>GAEPGARPPRIRIKTGIEVLKEQNFKCLEGKRVGLITNPTGVDNHLISTIDILHEAPNVNLVALYGPEHGVRGDVHAGDKVDNANDSSTGLPVYSLYGKTRKPTPEMLKDIDVLVYDIQDIGCRSFTYISTMGVAMEAAAENNKEFIVLDRPNPIGGLKIEGNVVEDGYISFVSQFKIPYLYGLTCGELALMLNGEQMLSKPCNLHVVKMKGWKRKMDYVQTGLQWIPSSPHIPHPHSAFFYPVSGILGELGYMSIGVGYTIPFQMFAARWVEAEKLADNLNRLHLPGVIFRPMHLKPFYSVGKEEHLQGVQVHIVDFNKASLSEIQFYVMQEVTALYPDRAVFDHADKERFHMFDLVSGSKEIRERFSQRNRWEDVRDYWY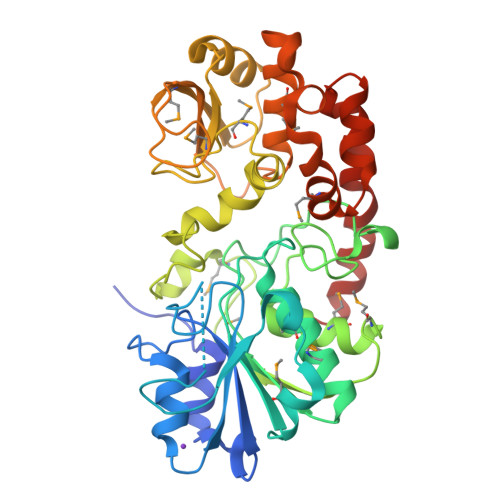KDVDDFRRLSQKYYLYK[2x]>[2x]EFARPCIPKS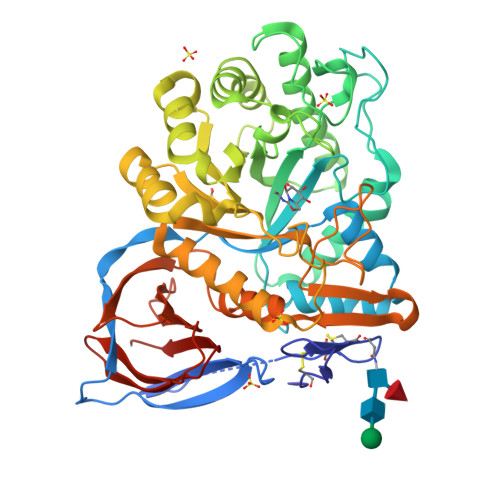FGYSSVVCVCNATYCDSFDPPTFPALGTFSRYESTRSGRRMELSMGPIQANHTGTGLLLTLQPEQKFQKVKGFGGAMTDAAALNILALSPPAQNLLLKSYFSEEGIGYNIIRVPMASCDFSIRTYTYADTPDDFQLHNFSLPEEDTKLKIPLIHRALQLAQRPVSLLASPWTSPTWLKTNGAVNGKGSLKGQPGDIYHQTWARYFVKFLDAYAEHKLQFWAVTAENEPSAGLLSGYPFQCLGFTPEHQRDFIARDLGPTLANSTHHNVRLLMLDDQRLLLPHWAKVVLTDPEAAKYVHGIAVHWYLDFLAPAKATLGETHRLFPNTMLFASEACVGSKFWEQSVRLGSWDRGMQYSHSIITNLLYHVVGWTDWNLALNPEGGPNWVRNFVDSPIIVDITKDTFYKQPMFYHLGHFSKFIPEGSQRVGLVASQKNDLDAVALMHPDGSAVVVVLNRSSKDVPLTIKDPAVGFLETISPGYSIHTYLWHRQLLVDTM> E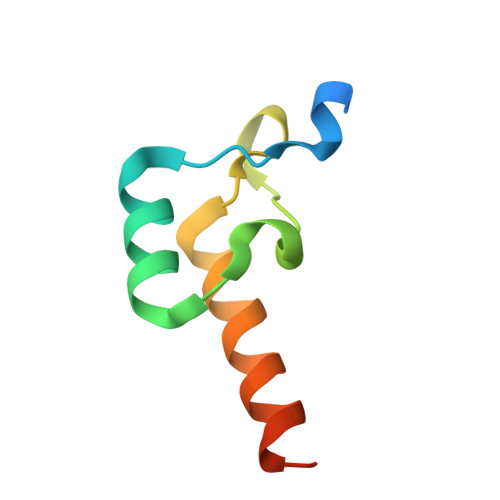GKSEFAENDAYVHATPLIRRLAREFGVNLAKVKGTGRKGRILREDVQAYVKEAIKRAEAAPAATG Enteroviruses particles are composed of single-strand RNA (virion RNA) genomes encapsulated by an icosahedral capsid of ~30 nm in diameter. In this study, we genetically perturb this equilibrium in a non-enveloped virus, enterovirus A71 to determine its structural basis. We isolate a single-point mutation variant with increased particle thermotolerance and decreased efficiency of cell entry. Using cryo-electron microscopy and molecular dynamics simulations, we determine that the thermostable native particles have acquired an expanded conformation that results in a significant increase in protein dynamics.

To understand how structural changes during the uncoating process are altered by the K162E mutation, purified capsid of WT and K162E were examined by cryogenic electron microscopy (cryo-EM). The native state of the WT particle was refined to a resolution of 3.3 Å using the gold-standard Fourier shell correlation cutoff of 0.143. The reconstructed WT particle had a high degree of cross-correlation (score of 0.883) when compared to the previously reported EV-A71 native structure (EMDB ID: 20766). We observed classic “jelly-roll” beta-barrels formed by VP1, VP2, and VP3. Within that structure, we observed electron density corresponding to tightly packed lipid moiety, known as “pocket factor”. The pocket factor in the WT particle interacts directly with the VP1 beta-barrel. Lysine 162 in VP1, well resolved in the density map, does not appear to interact with nearby residues. Instead, the positively charged side chain is exposed at the surface of the particle, near the exit site of the pocket factor. The exit site of the pocket factor is near K162, but the pocket-factor and K162 do not directly interact. A side view of the WT structure reveals a tight interaction of the extended VP4 with the internal surface of the capsomer and the external surface of the RNA (VP4 in yellow and RNA in orange).

> GDRVADVIESSIGDSVSRALTRALPAPTGQDTQVSSHRLDTGKVPALQAAEIGASSNASDESMIETRCVLNSHSTAETTLDSFFSRAGLVGEIDLPLEGTTNPNGYANWDIDITGYAQMRRKVELFTYMRFDAEFTFVACTPTGQVVPQLLQYMFVPPGAPKPDSRESLAWQTATNPSVFVKLSDPPAQVSVPFMSPASAYQWFYDGYPTFGEHKQEKDLEYGACPNNMMGTFSVRTVGTSKSKYPLVIRIYMRMKHVRAWIPRPMRNQNYLFKANPNYAGNFIKPTGASRTAITTL;> SPSAEACGYSDRVAQLTIGNSTITTQEAANIIVGYGEWPSYCSDSDATAVDKPTRPDVSVNRFYTLDTKLWEKSSKGWYWKFPDVLTETGVFGQNAQFHYLYRSGFCIHVQCNASKFHQGALLVAVLPEYVIGSVAGGTGTEDTHPPYKQTQPGADGFELQHPYVLDAGIPISQLTVCPHQWINLRTNNCATIIVPYINALPFDSALNHCNFGLLVVPISPLDYDQGATPVIPITITLAPMCSEFAGLRQAVTQ;> GFPTELKPGTNQFLTTDDGVSAPILPNFHPTPCIHIPGEVRNLLELCQVETILEVNNVPTNATSLMERLRFPVSAQAGKGELCAVFRADPGRSGPWQSTLLGQLCGYYTQWSGSLEVTFMFTGSFMATGKMLIAYTPPGGPLPKDRATAMLGTHVIWDFGLQSSVTLVIPWISNTHYRAHARDGVFDYYTTGLVSIWYQTNYVVPIGAPNTAYIIALAAAQKNFTMKLCKDASDILQTGTIQ;> MGSQVSTQRSGSHENSNSATEGSTINYTTINYYKDSYAATAGKQSLKQDPDKFANPVKDIFTEMAAPLK> MLADENDNHPLFTEGTYQAEVMENSPAGTPLTVLNGPILALDADEDVYAVVTYQLLGTHSDLFVIDNSTGVVTVRSGIIIDREAFSPPFLELLLLAEDIGQLNGTAHLFITILDDNDNWPTFSPPTYTVHLLENCPPGFSVLQVTATDEDSGLNGELVYRIEAGAQDRFLI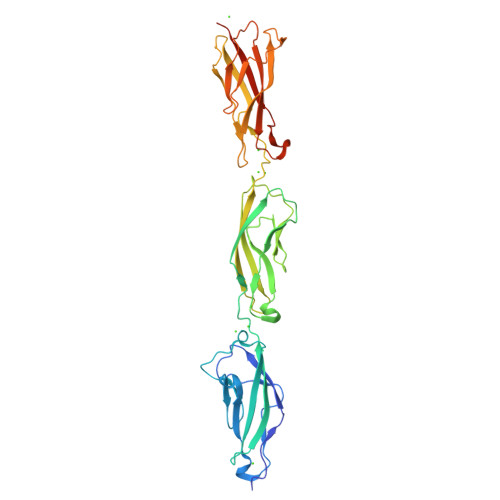HPVTGVIRVGNATIDREEQESYRLTVVATDRGTVPLSGTAIVTILIDDINDSRPEFLNPIQTVSVLESAEPGTIIANVTAIDLDLNPKLEYHIISIVAKDDTDRLVPDQEDAFAVNINTGSVMVKSPLNRELVATYEVTLSVIDNASDLPEHSVSVPNAKLTVNILDVNDNLEHHHHHH>[2x]KKSQYLEKINEVIRRAWAVPTHGHELGYSLCNSLRQSGGLDLLMKNCVKPDLQFSSAQLLEQCLTTENRKHVVDNGLDKVVNVACVCTKNSNMEHSRVGTGILEHLFKHSEGTCSDVIRLGGLDAVLFECRTSDLETLRHCASALANLSLYGGAENQEEMILRKVPMWLFPLAFHNDDNIKYYACLAIAVLVANKEIEAEVLKSGCLDLVEPFVTSHDPSAFARSNLAHAHGQSKHWLKRLVPVLSSNREEARNLAAFHFCMEAGIKREQGNTDIFREINAIEALKNVASCPNAIASKFAAQALRLIGET

Sterile alpha and TIR motif-containing protein 1 (SARM1) plays a central, pro-degenerative role in programmed axon death (including Wallerian degeneration). SARM1 has a critical nicotinamide adenine dinucleotide (NAD) cleavage (NADase) activity, which is activated when its upstream regulator and axon survival factor nicotinamide mononucleotide adenylyltransferase 2 (NMNAT2) is depleted or inactive (Essuman et al., 2017; Gilley et al., 2015; Gilley and Coleman, 2010; Sasaki et al., 2020a, Sasaki et al., 2016). Recent structural data revealed the existence of an allosteric pocket in SARM1 armadillo-repeat (ARM) domain which is important for the regulation of SARM1 activity. NMN binds to this pocket, leading to SARM1 activation.

Because we were unable to produce hSARM1ARM recombinantly, we used the ARM domain of Drosophila SARM1 (dSARM1ARM, residues 315–678), produced in E. coli, to investigate if VMN interacts directly with dSARM1ARM. Isothermal titration calorimetry (ITC) analysis showed that VMN bound to dSARM1ARM with a Kd value of 2.83 ± 0.16 μM (1:1 molar ratio). To further characterise this interaction, we determined the crystal structure of the VMN-bound dSARM1ARM (1.69 Å resolution). dSARM1ARM contains eight tandem armadillo repeats (ARM1-8) stacking into an unusually compact right-handed superhelix. The bound VMN molecule sits in the central groove of dSARM1ARM, which is mainly lined by the H3 helices from ARM1-5. The interaction is mediated by two pi-stacking interactions between the indole of W385 and the pyridine moiety of VMN, and between the imidazole ring of H392 and the nitrobenzene moiety of VMN; and eight hydrogen bonds, with a buried surface area of ~910 Å2. The hydroxyl group from the side chain of Y396 and the amino groups from the side chains of the conserved R437 and K476 form hydrogen bonds with the phosphate group of VMN; the amino group from the side chain of N640 forms a hydrogen bond with the nitro group of VMN; and the imidazole rings of H392 and H473 form hydrogen bonds with the urea and ribose of VMN, respectively. VMN-bound dSARM1ARM adopts a similar conformation to NMN-bound dSARM1ARM. Comparison of the two structures reveals that the NMN moiety of VMN and NMN share the same binding mode, with the key residues involved in NMN binding interacting with the analogous portions of the VMN molecule. Importantly, in the NMN-bound structure, NMN forms a hydrogen bond with the residues H599 and G600 (loop connecting ARM6 and 7), while in the VMN-bound structure, due to the extra portion of VMN (urea and nitrobenzene groups) extending to the region between the N- and C-termini of the protein, two different hydrogen bonds are formed between VMN and H392 (ARM2 H1) at the N-terminus, and N640 (ARM8 H1) at the C-terminus. Furthermore, the pi-stacking interaction between H392 and the nitrobenzene of VMN is specific to this compound.>[2x]MRNTKRAVVFAGDYAYIRQIETAMKSLCRHNSHLKIYLLNQDI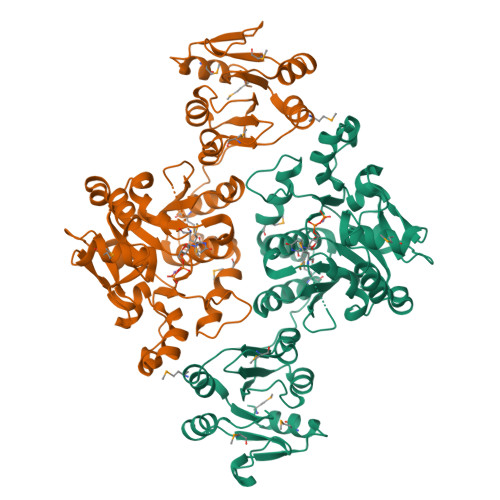PQEWFSQIRIYLQEMGGDLIDCKLIGSQFQMNWSNKLPHINHMTFARYFIPDFVTEDKVLYLDSDLIVTGDLTDLFELDLGENYLAAARSCFGAGVGFNAGVLLINNKKWGSETIRQKLIDLTEKEHENVEEGDQSILNMLFKDQYSSLEDQYNFQIGYDYGAATFKHQFIFDIPLEPLPLILHYISQDKPWNQFSVGRLREVWWEYSLMDWSVILNEWFSKSVKYPSKSQIFKLQCVNLTNSWCVEKIDYLAEQLPEVHFHIVAYTNMANELLALTRFPNVTVYPNSLPMLLEQIVIASDLYLDLNHDRKLEDAYEFVLKYKKPMIAFDNTCSENLSEISYEGIYPSSIPKKMVAAIRSYMR A virtually identical catalytic Asp-His-Ser triad was also found in rhamno­galacturonan acetylesterase (RGAE) and the esterase catalysis is assumed to follow a similar mechanism. Analysis of the structure of RGAE and comparison with structurally related enzymes led to the initial characterization of the SGNH-hydrolase family, which is now defined as a superfamily in SCOP. The structure of RGAE from Aspergillus aculeatus is known in two different crystal systems: a trigonal form and an orthorhombic form to very high (1.12 Å) resolution. An extremely low-field signal (at approximately 18 p.p.m.) in the 1H NMR spectrum of rhamnogalacturonan acetylesterase (RGAE) shows the presence of a short strong hydrogen bond in the structure.

In order to examine this hypothesis, a variant of RGAE was prepared in which the catalytic negatively charged Asp was replaced with an Asn. The crystal structure of RGAE D192N was determined to 1.33 Å resolution and refined to an R value of 11.6% for all data. The structure is virtually identical to the high-resolution (1.12 Å) structure of the wild-type enzyme except for the interactions involving the mutation and a disordered loop. The short Asp–His hydrogen bond observed in the wild type is not present and the corresponding distance between Asn192 and His195 is approximately 0.8 Å longer. As in wild-type RGAE, the imidazole group of His195 is hydrogen bonded to Ser9 (2.73 Å), whereas a hydrogen bond to a water molecule (2.79 Å) has replaced the hydrogen bond to Asp192. In RGAE D192N an acetate ion is bound in a similar position, with an O atom occupying the oxyanion hole almost in the same position as the O atom of the sulfate ion in wild-type RGAE. One loop (Gly77–Thr81) was poorly defined in the electron density of RGAE D192N. It is evident from the crystal packing that this loop cannot be in the same conformation as observed in the structure of the wild type and the disorder is most likely to be a result of differences in crystal packing and not a consequence of the D192N mutation. An analysis of the packing of RGAE D192N revealed that contacts involving Glu residues 94, 202 and 206 are similar to those of the trigonal wild-type form. Based on the structure of the D192N variant and the corresponding 1H NMR spectra we could rule out this active-site hydrogen bond as the sole origin of these signals, as the 18.2 p.p.m. signal persists in the spectra of RGAE D192N despite the mutation and the absence of the 14 p.p.m. signal in RGAE D192N.

> TTVYLAGDSTMAKNGGGSGTNGWGEYLASYLSATVVNDAVAGRSARSYTREGRFENIADVVTAGDYVIVEFGHNDGGSLSTDNGRTDCSGTGAEVCYSVYDGVNETILTFPAYLENAAKLFTAKGAKVILSSQTPNNPWETGTFVNSPTRFVEYAELAAEVAGVEYVDHWSYVDSIYETLGNATVNSYFPINHTHTSPAGAEVVAEAFLKAVVCTGTSLKSVLTTTSFEGTCL N-hydroxy-4-[(4-methylpiperazin-1-yl)methyl]benzamide | C13 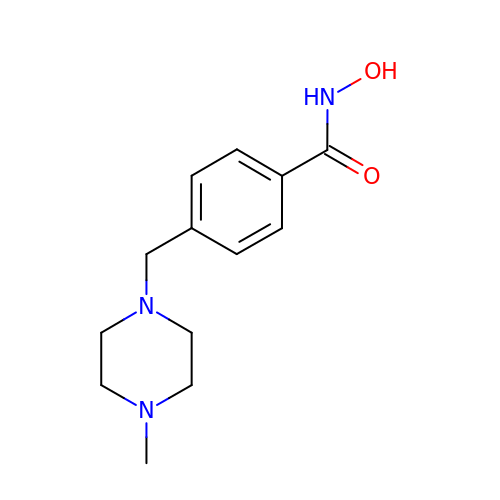H19 N3 O2 | VMDZCGSWWDTUMR-UHFFFAOYSA-N> MYGKIIFVLLLSEIVSISASSTTGVAMHTSTSSSVTKSYISSQTN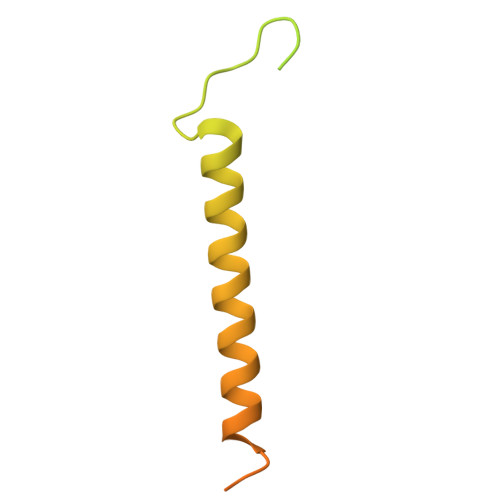DTHKRDTYAATPRAHEVSEISVRTVYPPEEETGERVQLAHHFSEPEITLIIFGVMAGVIGTILLISYGIRRLIKKSPSDVKPLPSPDTDVPLSSVEIENPETSDQ Enteroviruses particles are composed of single-strand RNA (virion RNA) genomes encapsulated by an icosahedral capsid of ~30 nm in diameter. In this study, we genetically perturb this equilibrium in a non-enveloped virus, enterovirus A71 to determine its structural basis. We isolate a single-point mutation variant with increased particle thermotolerance and decreased efficiency of cell entry. Using cryo-electron microscopy and molecular dynamics simulations, we determine that the thermostable native particles have acquired an expanded conformation that results in a significant increase in protein dynamics.

The population of K162E particles containing Coulomb potential, which correspond to viral RNA, at the center of the particle (A-particles) was heterogeneous in nature and composed of at least three distinct structures. The three states (A1, A2, A3) were resolved by 3D class averaging and refinement steps. The proportions of A1, A2, and A3 in the heat-inactivated preparation were 67.4%, 19.4%, and 7.9%, respectively. These structures were resolved at 3.1, 7.4, and 5.9 Å resolution for A1, A2, and A3, respectively. Interestingly, while the most abundant state A1 contained both VP4 and the pocket factor, A2 had lost the pocket factor but retained VP4, and A3 no longer contained pocket factor or VP4. A trajectory of irreversible molecule loss was resolved from the presence of either none, one, or both molecules. These data suggest that the pocket factor must be dislodged prior to VP4 loss, and both molecules must be released prior to complete genome uncoating. We observed a couple of intermediates that suggest that the first step in particle conversion is the release of the pocket factor (A1 particle to A2 particle), followed by large rearrangement of the N-terminus of VP1 and release of VP4 (A2 particle to A3 particle). Finally, virus RNA is expelled generating empty particles (A3 particle to empty particle).

> SHSTAETTLDSFFSRAGLVGEIDLPLEGTTNPNGYANWDIDITGYAQMRRKVELFTYMRFDAEFTFVACTPTGQVVPQLLQYMFVPPGAPEPDSRESLAWQTATNPSVFVKLSDPPAQVSVPFMSPASAYQWFYDGYPTFGEHKQEKDLEYGACPNNMMGTFSVRTVGTSKSKYPLVIRIYMRMKHVRAWIPRPMRNQNYLFKANPNYAGNFIKPTGASRTAITT;> LTIGNSTITTQEAANIIVGYGEWPSYCSDSDATAVDKPTRPDVSVNRFYTLDTKLWEKSSKGWYWKFPDVLTETGVFGQNAQFHYLYRSGFCIHVQCNASKFHQGALLVAVLPEYVIGTVAGGTGTEDSHPPYKQTQPGADGFELQHPYVLDAGIPISQLTVCPHQWINLRTNNCATIIVPYINALPFDSALNHCNFGLLVVPISPLDYDQGATPVIPITITLAPMCSEFAGLRQ;> GFPTELKPGTNQFLTTDDGVSAPILPNFHPTPCIHIPGEVRNLLELCQVETILEVNNVPTNATSLMERLRFPVSAQAGKGELCAVFRADPGRSGPWQSTLLGQLCGYYTQWSGSLEVTFMFTGSFMATGKMLIAYTPPGGPLPKDRATAMLGTHVIWDFGLQSSVTLVIPWISNTHYRAHARDGVFDYYTTGLVSIWYQTNYVVPIGAPNTAYIIALAAAQKNFTMQLCKDASDIL> MAAETASGYIQHHLQNLTFGRLPNGDWGFAHTAEQAKEMGFWAFHVDTLGWSVLLGVVFLFIFRLAAKKATSGQPGGLQNFVEVMVEFVDTSVKDTFHGRNP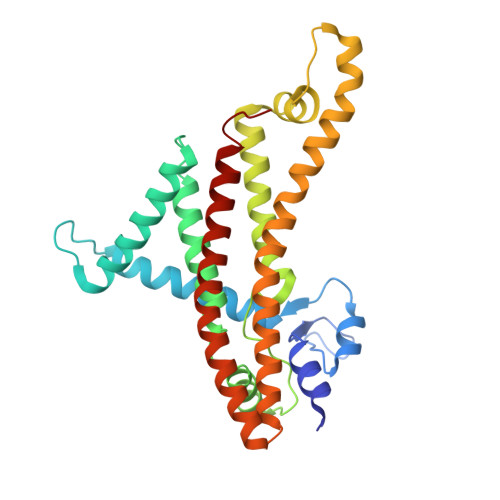LIAPLALTVFVWIFLLNLIDLVPVDYLPMLAAKITGDEHLFFRAVATTDPNATLGLSISVFALIVFYSIKVKGIGGFLGELTLHPFSSKNIVVQILLIPVNFLLEFVTLIAKPVSLALRLFGNMYAGELIFILIAVMFGSGMFLLSALGVALNWAWAVFHILIITLQAFIFMMLTIVYLSMAHEDNH> IVQQFRIYSNELIMKHDRHERIVKLSRDITIESKRIIFLLHSIDSRKQNKEKVLEEARQRLNKLIAVNFRAVALELRDQDVYQFRSSYSPGLQEFIEAYTYMEYLCHEDAEGENETKSVSDWQAIQAVMQYVEESSQPKEEPTEGEDVQAIAQVESPKKFQFFVDPTEYILGLSDLTGELMRRCINSLGSGDTDTCLDTCKALQHFYSGYISLNCQRARELWRKITTMKQSVLKAENVCYNVKVRGGEAAKWGATFDQKPADEV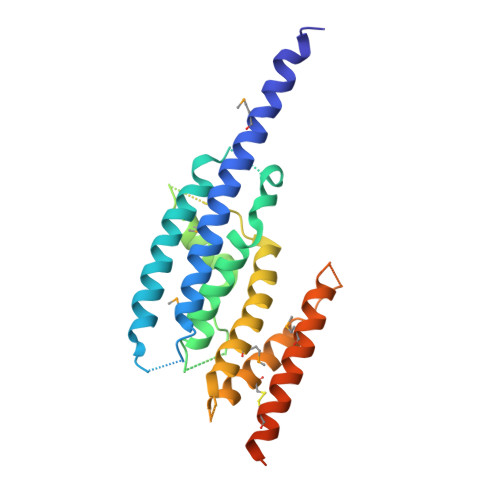DEGFY>[2x]ETGDEDLPGAVPTESIQGSTFEEKIFLQWREPTQTYGVITLYEITYKAVSSFDPEIDLSNQSGRVSKLGNETHFLFFGLYPGTTYSFTIRASTAKGFGPPATNQFTTKISAPSMPAYELETPLNQTDNTVTVMLKPAHSRGAPVSVYQIVVEEERPRRTKKTTEILKCYPVPIHFQNASLLNSQYYFAAEFPADSLQAAQPFTIGDNKTYNGYWNTPLLPYKSYRIYFQAASRANGETKIDCVQVATKGGTKHHHHHH

Type IIB receptor protein tyrosine phosphatases are cell surface transmembrane proteins that engage in cell adhesion via their extracellular domains (ECDs) and cell signaling via their cytoplasmic phosphatase domains. The four human R2B RPTPs (PTPRK, PTPRM, PTPRT, and PTPRU) are type 1 transmembrane proteins and share a common extracellular domain (ECD) architecture of one MAM (meprin/A5/μ), one immunoglobulin (Ig)-like, and four fibronectin (FN) type-III domains, with the most membrane proximal FN domain undergoing furin cleavage in the secretory pathway. Previous studies have shown that PTPRK, PTPRM, and PTPRT form homodimers, but not heterodimers, in cell aggregation assays. The homophilic (trans) interactions of R2B RPTPs determine their subcellular localization and have been proposed to function as spacer clamps between cell membranes.

Crystals grew in two space groups, P212121 and P3221, possessing two and four molecules per asymmetric unit, respectively. All six chains are essentially identical in structure (pairwise RMSDs over 220 Cα atoms range from 0.44 to 0.92 Å). The main difference between the protein structures is that one chain in the P212121 crystal has a disordered loop (residues 628–641) that in all other chains was ordered via intermolecular interactions. This loop is anchored at one end via a disulfide bond within the FN4 domain (C642 to C716), and the sequence encompasses the furin-cleavage site of PTPRM, illustrating that this site is surface accessible within a conformationally dynamic loop, but that cleavage would not significantly destabilize the fold of the FN4 domain. In both crystal forms, one chain is missing the glycan on N598, indicating that PTPRM-FN4 not only adopts conformational differences in the furin-cleavage loop but also can undergo heterogeneous glycosylation. Although the previous structure of the PTPRM ECD had no interpretable electron density for the FN4 domain, it was present in the construct. Superposition of the FN3 domains from our structure with this previous PTPRM structure demonstrates that the FN4 domain can be accommodated without significant steric clashes with surrounding chains, and FN4 colocalizes with weak and disconnected electron density that is unmodeled in the deposited structure.Pygo and BCL9/Legless transduce the Wnt signal by promoting the transcriptional activity of β-catenin/Armadillo in normal and malignant cells. Molecularly, BCL9/Lgs proteins function as adaptors between Pygo and Armadillo/β-catenin, by binding through their homology domain 1 (HD1) to the PHD finger in the C terminus of Pygo, and through their homology domain 2 (HD2) to the Armadillo repeat domain of Armadillo/β-catenin (Kramps et al., 2002; Städeli and Basler, 2005). We show that human and Drosophila Pygo PHD fingers associate with their cognate HD1 domains from BCL9/Legless to bind specifically to the histone H3 tail methylated at lysine 4 (H3K4me). Therefore, this is a prime example of histone tail binding by a PHD finger (of Pygo) being modulated by a cofactor (BCL9/Legless).

In one of our PHD-HD1 crystals (space group C2221, WT2), where two binary complexes are seen in the asymmetric unit, one of the N-terminal hPHD ends was inserted into the peptide-binding pocket of the second complex, thus behaving as a pseudoligand. The structure of the free hPHD finger (Nakamura et al., 2007) shows a dimer in the crystal, in which the PHD-PHD interaction mimics the PHD-HD1 interaction that we see. This PHD-PHD interaction may thus merely reflect a propensity of the hydrophobic loop2 surface to undergo a pseudoligand interaction in the absence of bona fide ligand, similar to the pseudoligand interaction we observed between the hPHD N terminus and the H3K4me-binding pocket.

>MGHSSSDPVYPCGICTNEVNDDQDAILCEASCQKWFHRICTGMTETAYGLLTAEASAVWGCDTCMAD[2x];>[2x]AMAAKVVYVFSTEMANKAAEAVLKGQVETIVSFHI Akkermansia muciniphila is an anaerobic intestinal commensal bacterium which possesses specific β-N-acetylhexosaminidases for gut mucosal layer colonization and mucin degradation. In this study, we assessed the in vitro mucin glycan cleavage activity of the A. muciniphila β-N-acetylhexosaminidase Am2136 and demonstrated its ability that hydrolyzing the β-linkages joining N-acetylglucosamine to a wide variety of aglycone residues, which indicated that Am2136 may be a generalist β-N-acetylhexosaminidase. The GH20 family has the largest number of β-N-acetylhexosaminidases, and they generally utilize the substrate-assisted mechanism. Among the known GH20 family members, Am2136 is unique for its possession of additional N-terminal domain (D21-G107) and C-terminal galectin-like domain (D601-L756).20 The galectin-like domain usually acts as a sugar moiety-recognition module.

The crystal structure of Am2136 (without signal peptide residues 1–19) in apo form was solved to 2.9 Å. Am2136 consists of four domains, in which the central II and III domains correspond to GH20b and GH20 domains separately. The catalytic domain III was flanked by domain I, II and IV, in which the majority of interdomain contacts were established by the galectin-like domain IV (1099.1 Å2). This galectin-like module adopts a closing hand shape formed by two antiparallel β-sheet sandwiches (β23-β33). It forms several hydrogen bonds (R665-G546/Y547, R730-T545) and a charge–charge interaction (K714-D717) with domain III, by which the extended V-type loop (V707-T732) can participate in the substrate-binding pocket formation. Hence, these results demonstrate that the specific interactions between domain III and IV are an important integral part of regulating the hydrolysis activity. The residue E413 provides a proton to the aglycone leaving group during the oxazolinium formation step, and then abstract one from the nucleophilic water during the oxazolinium hydrolysis, while D412 stabilizes the oxazolinium intermediate. Thus, Y415 is a crucial part of the hydrophobic pocket necessary for substrate binding, this interpretation is further supported by the obvious increased Km value (2.32 mM) of mutant Y415A. According to molecule docking calculations, the most probable nucleotide-binding site of Am2136 is found in the cleft between domain III and IV, located at more than 28.6 Å from the active site. Five critical residues (S249, K252, R256, Y550, E649) that form direct interactions with GDP.

> QDAKQIADSLSIPPVKAGAKQLPMPSVSGAQIKLLGADYEQLVNSKGKIAPVISDTPVNVSFKVTKDGKEAVSKDYEIMLQAPQAAQGNPKPRIIPEILQWKGGQGEYKLGNTVTIACPDKELGKLFAADMEDVLGKKVKLVAPGAKADISLSLLKGGNLGREGYRLQIARDGVRLGAAAPTGLFWGTRTLLQMLRQTPGSVPCGTAVDFPRYQLRGFMLDVARTPYPLSYLKDVIRTMAWYKMNDLHLVINNNYIFHEHYVDNGHDPFKESYAAFRLESKMKGKDGTPLTARDLFYTKKEFADLVSYARKYGVNIVPEFDTPGHALSFTRLRPDLIYKGPMNHEKRRCEMLDAANPETIDLVSKVFDEYMLKDPKLGRPVFADCGVVHVGADEFYGDKEDYRHFANAVLTHALKRGYTPRIWGSLSAKPGKTPVVSKGVQMNLWSTGWMKAWEAVNQGYDVINTNDGALYIVPFAGYYRMDRNHKGLYNNWIPNRIGNETLPSGHPQLLGGTFAVWNDETDIMHTGYAPYDIWGIISGSMDVLSQKLWGTAKAPDTFEQHRELVSSIGNAPRTNPLHKWKDSQPLTVKPSSLPQKLDKPALGPNYRLTMELELTAAPEGKEQVLLAAPEGELLAVMKDGTVGFRRDDSLEFSFGAKLPVGKKVKVEIVGEPEKTSLLLDGEPAGTAVLKNFSDKSKDFSDKFKHRPKVHRSTFILPLKELGSSFQGKVFHMNVQPL;> SIPPVKAGAKQLPMPSVSGAQIKLLGADYEQLVNSKGKIAPVISDTPVNVSFKVTKDGKEAVSKDYEIMLQAPQAAQGNPKPRIIPEILQWKGGQGEYKLGNTVTIACPDKELGKLFAADMEDVLGKKVKLVAPGAKADISLSLLKGGNLGREGYRLQIARDGVRLGAAAPTGLFWGTRTLLQMLRQTPGSVPCGTAVDFPRYQLRGFMLDVARTPYPLSYLKDVIRTMAWYKMNDLHLVINNNYIFHEHYVDNGHDPFKESYAAFRLESKMKGKDGTPLTARDLFYTKKEFADLVSYARKYGVNIVPEFDTPGHALSFTRLRPDLIYKGPMNHEKRRCEMLDAANPETIDLVSKVFDEYMLKDPKLGRPVFADCGVVHVGADEFYGDKEDYRHFANAVLTHALKRGYTPRIWGSLSAKPGKTPVVSKGVQMNLWSTGWMKAWEAVNQGYDVINTNDGALYIVPFAGYYRMDRNHKGLYNNWIPNRIGNETLPSGHPQLLGGTFAVWNDETDIMHTGYAPYDIWGIISGSMDVLSQKLWGTAKAPDTFEQHRELVSSIGNAPRTNPLHKWKDSQPLTVKPSSLPQKLDKPALGPNYRLTMELELTAAPEGKEQVLLAAPEGELLAVMKDGTVGFRRDDSLEFSFGAKLPVGKKVKVEIVGEPEKTSLLLDGEPAGTAVLKNFSDKSKDFSDKFKHRPKVHRSTFILPLKELGSSFQGKVFHMNVQPL;> ADSLSIPPVKAGAKQLPMPSVSGAQIKLLGADYEQLVNSKGKIAPVISDTPVNVSFKVTKDGKEAVSKDYEIMLQAPQAAQGNPKPRIIPEILQWKGGQGEYKLGNTVTIACPDKELGKLFAADMEDVLGKKVKLVAPGAKADISLSLLKGGNLGREGYRLQIARDGVRLGAAAPTGLFWGTRTLLQMLRQTPGSVPCGTAVDFPRYQLRGFMLDVARTPYPLSYLKDVIRTMAWYKMNDLHLVINNNYIFHEHYVDNGHDPFKESYAAFRLESKMKGKDGTPLTARDLFYTKKEFADLVSYARKYGVNIVPEFDTPGHALSFTRLRPDLIYKGPMNHEKRRCEMLDAANPETIDLVSKVFDEYMLKDPKLGRPVFADCGVVHVGADEFYGDKEDYRHFANAVLTHALKRGYTPRIWGSLSAKPGKTPVVSKGVQMNLWSTGWMKAWEAVNQGYDVINTNDGALYIVPFAGYYRMDRNHKGLYNNWIPNRIGNETLPSGHPQLLGGTFAVWNDETDIMHTGYAPYDIWGIISGSMDVLSQKLWGTAKAPDTFEQHRELVSSIGNAPRTNPLHKWKDSQPLTVKPSSLPQKLDKPALGPNYRLTMELELTAAPEGKEQVLLAAPEGELLAVMKDGTVGFRRDDSLEFSFGAKLPVGKKVKVEIVGEPEKTSLLLDGEPAGTAVLKNFSDKSKDFSDKFKHRPKVHRSTFILPLKELGSSFQGKVFHMNVQPL;> KQIADSLSIPPVKAGAKQLPMPSVSGAQIKLLGADYEQLVNSKGKIAPVISDTPVNVSFKVTKDGKEAVSKDYEIMLQAPQAAQGNPKPRIIPEILQWKGGQGEYKLGNTVTIACPDKELGKLFAADMEDVLGKKVKLVAPGAKADISLSLLKGGNLGREGYRLQIARDGVRLGAAAPTGLFWGTRTLLQMLRQTPGSVPCGTAVDFPRYQLRGFMLDVARTPYPLSYLKDVIRTMAWYKMNDLHLVINNNYIFHEHYVDNGHDPFKESYAAFRLESKMKGKDGTPLTARDLFYTKKEFADLVSYARKYGVNIVPEFDTPGHALSFTRLRPDLIYKGPMNHEKRRCEMLDAANPETIDLVSKVFDEYMLKDPKLGRPVFADCGVVHVGADEFYGDKEDYRHFANAVLTHALKRGYTPRIWGSLSAKPGKTPVVSKGVQMNLWSTGWMKAWEAVNQGYDVINTNDGALYIVPFAGYYRMDRNHKGLYNNWIPNRIGNETLPSGHPQLLGGTFAVWNDETDIMHTGYAPYDIWGIISGSMDVLSQKLWGTAKAPDTFEQHRELVSSIGNAPRTNPLHKWKDSQPLTVKPSSLPQKLDKPALGPNYRLTMELELTAAPEGKEQVLLAAPEGELLAVMKDGTVGFRRDDSLEFSFGAKLPVGKKVKVEIVGEPEKTSLLLDGEPAGTAVLKNFSDKSKDFSDKFKHRPKVHRSTFILPLKELGSSFQGKVFHMNVQPL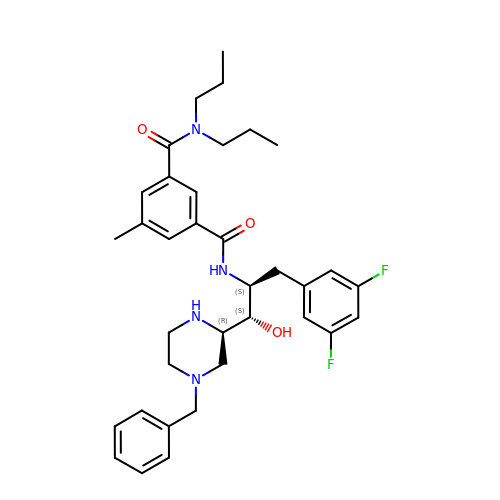N'-[(1S,2S)-2-[(2R)-4-benzylpiperazin-2-yl]-1-(3,5-difluorobenzyl)-2-hydroxyethyl]-5-methyl-N,N-dipropylbenzene-1,3-dicarboxamide | C35 H44 F2 N4 O3 | ZHZSBUKNHGZRTJ-DSPMFFIESA-N4-chloranyl-N-[(1R)-1-[(1S,5R)-3-quinolin-4-yloxy-6-bicyclo[3.1.0]hexanyl]propyl]benzamide 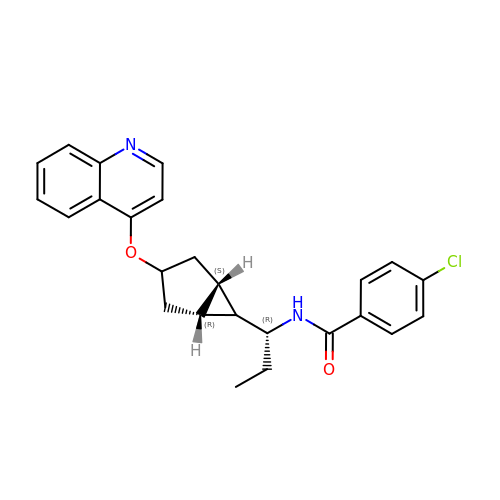| C25 H25 Cl N2 O2 | UAXPPQPDGOMVPD-MJALHYBGSA-N>GPGSLSQASADLEATLRHKLTVMYSQINGASRALDDVRNRQQDVRMTANRKVEQLQQEYTEMKALLDASETTSTRKIKEEEKRVNSKFDTIYQILLKKKSEIQTLKEEIEQSLTKRDEFEFLEKASKLRGISTKPVYIPEVELNHKLIKGIHQSTIDLKNELKQCIGRLQELTPSSGDPGEHDPASTHKSTRP[4x];>GPGMDPNTVSSFQVDCFLWHVRKRVADQELGDAPFLDRLRADQASLRGRGSTLGLDIETATRAGKQIVERILKEESDEALKMTMASVPASRYLTDMTLEEMSREWSMLIPKQKVAGPLCIRMDQAIMDKNIILKANFSVIFDRLETLILLRAFTEEGAIVGEISPLPSLPGHTAEDVKNAVGVLIGGLEANDNTVRVSETLQRFAWRSSNENGRPPLTPKQKREMAGTIRSEV[4x]

Tripartite motif (TRIM) family proteins are RING-type E3 ligases that play key regulatory roles in innate immune signalling pathways that lead to the induction of a type I interferon (IFN) response and production of inflammatory cytokines through activation of the IRF3 and NF-κB transcription factors. Activation of RIG-I initiates a signalling cascade that depends on the E3 ligase activity of TRIM25 and induces the production of IFNs and inflammatory cytokines. An example is non-structural protein 1 (NS1) of influenza A viruses (IAV), a multifunctional virulence factor that binds many host proteins during infection, including TRIM2527–29. To understand NS1-mediated inhibition of TRIM25 activity on a molecular level we have determined crystal structures of the CC domain of TRIM25 in complex with NS1-FL and the isolated ED, and of a TRIM25 CC-PRYSPRY fragment, which includes the RIG-I-recognition domain of TRIM25.

While our experiments established that the effector domain of NS1 is sufficient to form a stable complex with TRIM25, we wondered how the constraints imposed by the constitutively dimeric RBD within full-length NS1 might influence the architecture of the NS1/TRIM25 assembly. To gain insight into this arrangement we crystallised a complex between TRIM25-CC and the triple mutant NS1-FL (R38A/K41A/W187A) and solved the structure by molecular replacement at 4.26 Å resolution (R/Rfree = 0.27/0.31). Interestingly, the two NS1 monomers within the homodimer are not symmetrical; while both monomers align well on the NS1-RBD (RMSD of 0.6 Å), one NS1-ED is shifted towards the stem in relation to the other by ~17 Å. The relative arrangement of RBD and ED seen in this structure is different from previous structures of NS1-FL, supporting the model that the linker region acts as a flexible hinge to allow movement of the ED relative to the RBD to accommodate binding of different substrates. The only contacts between TRIM25-CC and NS1-FL are made by the ED, in agreement with our BLI experiments. Structural superposition of the NS1-ED/TRIM25-CC complex with that of NS1-FL/TRIM25-CC shows that interface A, but not interface B, is present in the full-length complex (RMSD 0.7 Å), confirming its physiological relevance. However, dimerisation is unperturbed in both TRIM25/NS1 complexes and instead the dimeric CC is recognised by two NS1 effector domains at its distal ends in a symmetrical fashion. Furthermore, a key observation from the NS1-FL/TRIM25-CC structure is that although the overall architecture of the complex is identical to that of NS1-ED/TRIM25-CC, the two EDs of a given NS1 homodimer bridge two different TRIM25 dimers that are located in a perpendicular arrangement in the crystal. We hypothesise that this arrangement highlights the critical role of the constitutive NS1-RBD dimer in mediating higher order oligomerization of the NS1–TRIM25 complex, which is likely important for the proviral function of NS1.> 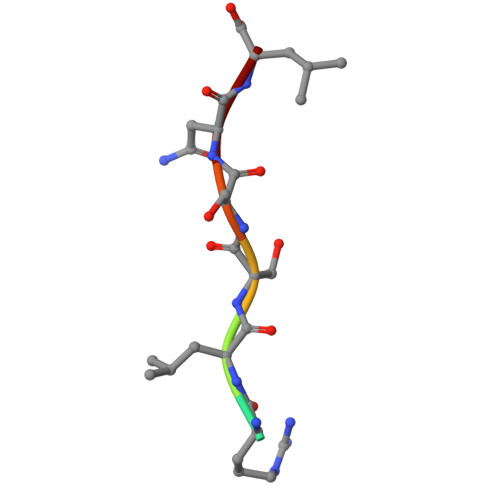SRLSSNL>MGSSHHHHHHSQDPNSAAPAAEAPLSHVQQALAELAKPKDDPTRKHVCVQVAPAVRVAIAETLGLAPGATTPKQLAEGLRRLGFDEVFDTLFGADLTIMEEGSELLHRLTEHLEAHPHSDEPLPMFTSCCPGWIAMLEKSYPDLIPYVSSCKSPQMMLAAMVKSYLAEKKGIAPKDMVMVSIMPCTRKQSEADRDWFCVDADPTLRQLDHVITTVELGNIFKERGINLAELPEGEWDNPMGVGSGAGVLFGTTGGVMEAALRTAYELFTGTPLPRLSLSEVRGMDGIKETNITMVPAPGSKFEELLKHRAAARAEAAAHGTPGPLAWDGGAGFTSEDGRGGITLRVAVANGLGNAKKLITKMQAGEAKYDFVEIMACPAGCVGGGGQPRSTDKAITQKRQAALYNLDEKSTLRRSHENPSIRE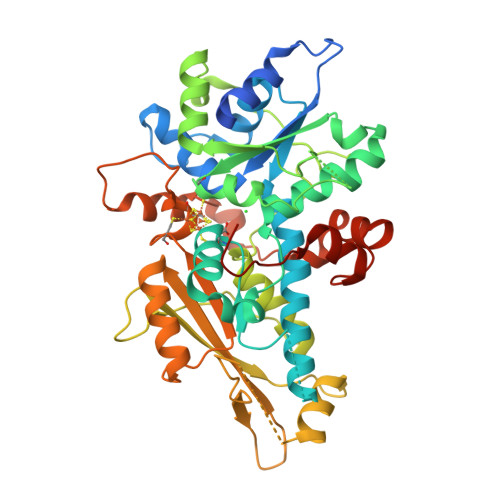LYDTYLGEPLGHKAHELLHTHYVAGGVEEKDEKK[2x]>[2x]GAASMSDDLVKILVLGPSKSGKSTVTNFLAGTRDTPTKEYHETNPLRVLE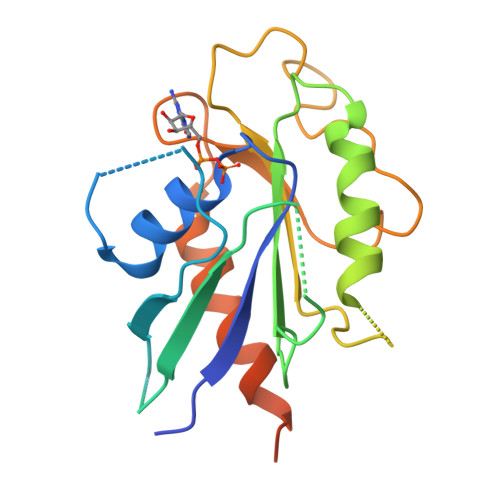VEIALDDTRRSGRQAAGLKKAVVQLWDVGGSSKHQAGWPAIASNADGIIYVFNPEVKGSEKELLLWYKNFALNQDELDDDNNFKMRVTDGHSLIFSHHSSLPEFAVGDNAIPPMPKQLQGIRALETSLDYQSDNFKEAFDALVEQIIASRLAAEENDLLQKEREAKDYPRLKR> RKSRY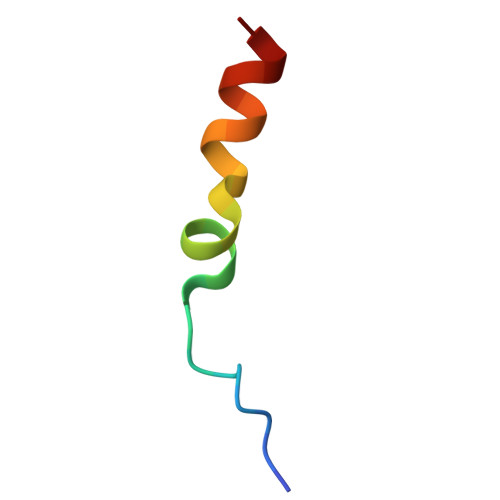AELDFEKIMHTRKRHQDMFQ> MIVIFVDFDYFFAQVEEVLNPQYKGKPLVVCVYSGRTKTSGAVATANYEARKLGVKAGMPIIKAMQIAPSAIYVPMRKPIYEAFSNRIMNLLNKHADKIEVASIDEAYLDVTNKVEGNFENGIELARKIKQEILEKEKITVTVGVAPNKILAKIIADKSKPNGLGVIRPTEVQDFLNELDIDEIPGIGSVLARRLNELGIQKLRDILSKNYNELEKITGKAKALYLLKLAQNKYSEPVENKSKIPHGRYLT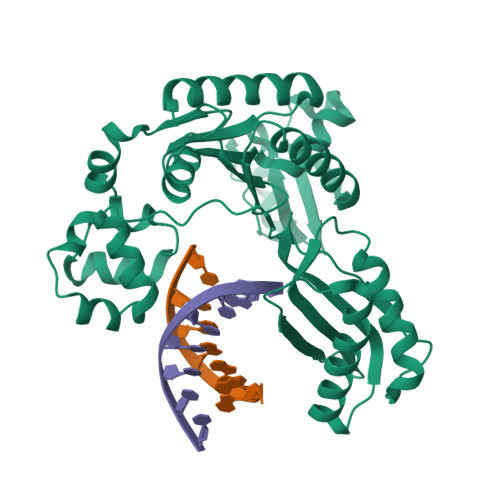LPYNTRDVKVILPYLKKAINEAYNKVNGIPMRITVIAIMEDLDILSKGKKFKHGISIDNAYKVAEDLLRELLVRDKRRNVRRIGVKLDNIIINKTNLSDFFDI3-borono-5-{[(thiophen-2-yl)acetyl]amino}benzoic acid | C13 H12 B N O5 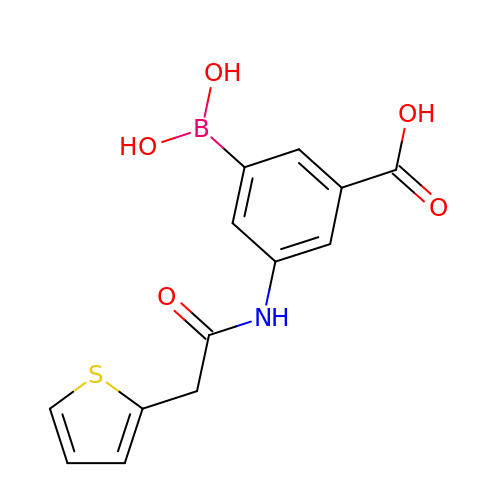S | CFVZHOLBBPQSIQ-UHFFFAOYSA-N>[5x]TDGAVTTSQIPASEQETLVRPKPLLLKLLKSVGAQKDTY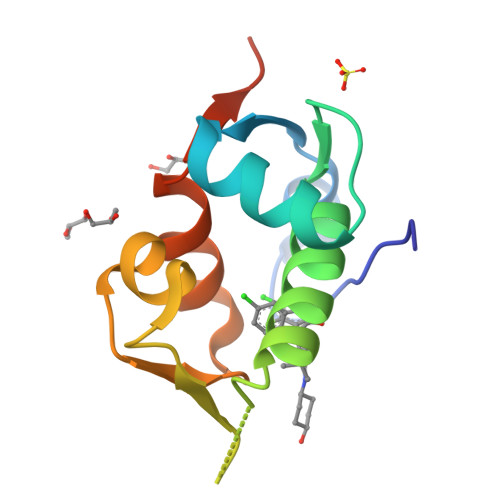TMKEVLFYLGQYIMTKRLYDEKQQHIVYCSNDLLGDLFGVPSFSVKEHRKIYTMIYRNLVVVNQQESSDS> 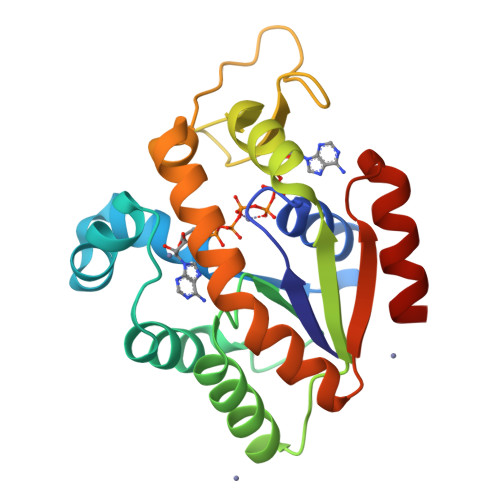MILVFLGPPGAGKGTQAKRLAKEKGFVHISTGDILREAVQKGTPLGKKAKEYMERGELVPDDLIIALIEEVFPKHGNVIFDGFPRTVKQAEALDEMLEKKGLKVDHVLLFEVPDEVVIERLSGRRINPETGEVYHVKYNPPPPGVKVIQREDDKPEVIKKRLEVYREQTAPLIEYYKKKGILRIIDASKPVEEVYRQVLEVIGDGN>[4x]MLVAGSELPRRPLPPAAQERDAEPRPPHGELQYLGQIQHILRCGVRKDDRTGTGTLSVFGMQARYSLRDEFPLLTTKRVFWKGVLEELLWFIKGSTNAKELSSKGVKIWDANGSRDFLDSLGFSTREEGDLGPVYGFQWRHFGAEYRDMESDYSGQGVDQLQRVIDTIKTNPDDRRIIMCAWNPRDLPLMALPPCHALCQFYVVNSELSCQL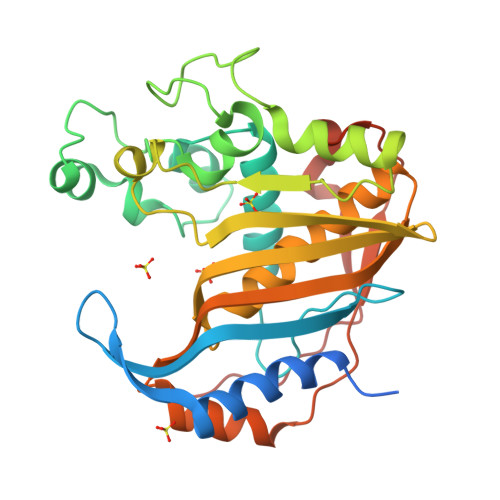YQRSGDMGLGVPFNIASYALLTYMIAHITGLKPGDFIHTLGDAHIYLNHIEPLKIQLQREPRPFPKLRILRKVEKIDDFKAEDFQIEGYNPHPTIKMEMAV>[6x]MATAQSNSPRVFCIGTADTKFDELRFLSEHVRSSLNSFSNKSSFKVGVTVVDVSTSWKETNSCADFDFVPSKDVLSCHTLGEETMGTFADIRGLA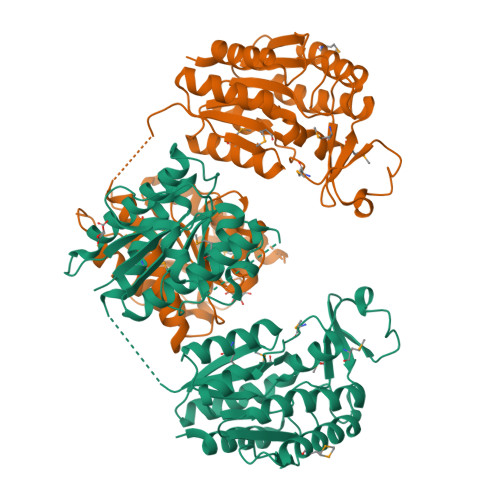IAIMSKALETFLSIANDEQNLAGVIGLGGSGGTSLLSSAFRSLPIGIPKVIISTVASGQTESYIGTSDLVLFPSVVDICGINNVSKVVLSNAGAAFAGMVIGRLESSKEHSITNGKFTVGVTMFGVTTPCVNAVKERLVKEGYETLVFHATGVGGRAMEDLVRGGFIQGVLDITTTEVADYVVGGVMACDSSRFDAILEKKIPLVLSVGALDMVNFGPKTTIPPEFQQRKIHEHNEQVSLMRTTVGENKKFAAFIAEKLNKASSSVCVCLPEKGVSALDAPGKDFYDPEATSCLTRELQMLLENNERCQVKVLPYHINDAEFANALVDSFLEISPK>SYTLPSLPYAYDALEPHFDKQTMEIHHTKHHQTYVNNANAALESLPEFANLPVEELITKLDQLPADKKTVLRNNAGGHANHSLFWKGLKKGTTLQGDLKAAIERDFGSVDNFKAEFEKAAASRFGSGWAWLV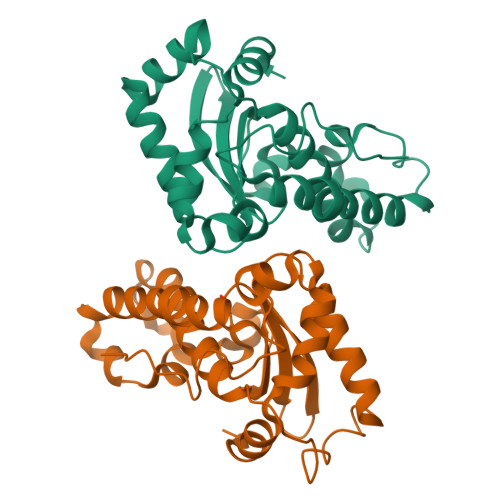LKGDKLAVVSTANQDSPLMGEAISGASGFPIMGLDVWEHAYYLKFQNRRPDYIKEFWNVVNWDEAAARFAAKK[4x]nonyl(oxo)di(propan-2-yl)-lambda~5~-phosphane | C15 H33 O P | 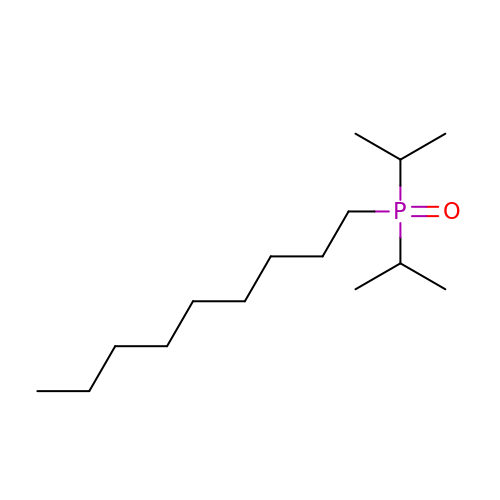DHOTYMJGZIUWRT-UHFFFAOYSA-N> MELKHSISDYTEAEFLEFVKKIEDANSSEDEQQKLVEEFIRLTEHPSGSDLIYYPRDDREDSPEGIVKEIKEWRAANGKSGFKQGLEHHHHHH;> MESKRNKPGKATGKGKPVGDKWLDDAGKDSGAPIPDRIADKLRDKEFKNFDDFRKKFWEEVSKDPDLAKQFKRSNRKRIQQGYAPFAPQKDQVGGRTTFELHHDKPISQDGGVYDMNNIRVTTPKRAIDIHRGK

The colE proteins are nonspecific DNases, which are produced by Escherichia coli to eliminate neighboring bacteria. To avoid autotoxicity, the producing cells co-express Im proteins, which tightly bind and inhibit colE’s activity. In the colE/Im system, comprising four homologous pairs (colEwt2/Imwt2, colEwt7/Imwt7, colEwt8/Imwt8, and colEwt9/Imwt9), each cognate pair forms an ultrahigh affinity complex (KD < 10−13 M), whereas the non-cognate pairs show non-protective affinities (KD > 10−10 M). Our results demonstrate that the design of substantially different backbone conformations, orientations, and sequences at the binding site generates dozens of new interaction pairs from a single starting one.

To verify the atomic accuracy of the design procedure, we determined the structures of two designed pairs by X-ray crystallography: colEdes3/Imdes3 with >3 orders of magnitude pairwise specificity relative to the wild-type colEwt2/Imwt2 and colEdes7/Imdes7 with low Im specificity. In both structures, the conserved hotspot region formed as predicted. For example, colEdes7/Imdes7 exhibited relatively high cognate affinity (51 nM), but Imdes7 bound three non-cognate colE proteins with similar or up to two orders of magnitude higher affinities. In the multispecific colEdes7/Imdes7, however, we noted a conformational change in loop I localized around Ala25, while the rest of the loop was atomically accurate (0.7 Å Cα rmsd on all Im side chains). Nevertheless, this local difference relative to the design conception prevented the formation of a designed hydrogen-bond network. Finally, backbone flexibility may disrupt the formation of the designed polar interactions, as seen in the crystal structure of colEdes7/Imdes7, enabling alternative binding modes and leading to multispecific molecular recognition as for Imdes7. By contrast, multispecific designs, such as Imdes6 and Imdes7, exhibited low Z-scores (1.4 and 1.5, respectively), including, in some cases, alternative backbone conformations of lower energy than the designed conformation. Imdes6, Imdes7, and Imdes8, by contrast, exhibit α1nM values <0.1 and are expected to bind multiple colE proteins at this concentration.heptyl 4-deoxy-4-deoxy-alpha-D-mannopyranoside 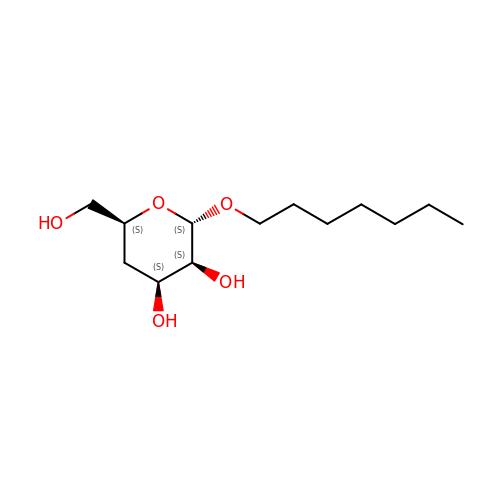| C13 H26 O5 | JEMWDTFNPZXRJX-CYDGBPFRSA-N> LKESPSGY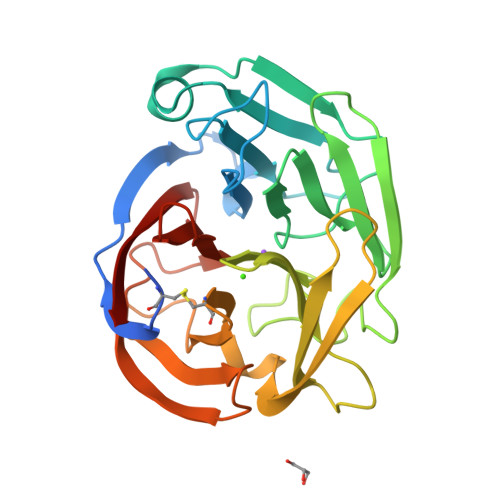LRSGEGDTGCGELVWVGEPLTLRTAETITGKYGVWMRDPKPTYPYTQETTWRIDTVGTDVRQVFEYDLISQFMQGYPSKVHILPRPLESTGAVVYSGSLYFQGAESRTVIRYELNTETVKAEKEIPGAGYHGQFPYSWGGYTDIDLAVDEAGLWVIYSTDEAKGAIVLSKLNPENLELEQTWETNIRKQSVANAFIICGTLYTVSSYTSADATINFAYDTGTGISKTLTIPFKNRYKYSSMIDYNPLEKKLFAWDNLNMVTYDIKLSKM> MTSHRQSSDTFGGILPSTLSSRYLSIVNQLPEEFSSVVSEMMVHLENIFSLAENFFQAIERFSRTPDLLERNKMSIGVGAEGDSWPCHVSHEAPMGSAQTTENSAKEEDKQVPESAALQHPKFKSTPGPQLPTRRRFLSESDELQDPQPVWDAEPQFCQGFLIQGLWELFMDSRQKNQQEHGGEDSSQESKDSGLCDFKPEPQPRHRNSLSDSADPFLIKSPSALLDYYQEDVSRPQPETQESSGRADKFLKPLSWGSEVLESSCNQPSTALWQLERFTVPQALQKVRVLKHQELLLVVAVSSFTRHVFTCSQSGIKVWNLVNQVAEDRDPESHLKCSVQDNKVYLRTCLLSSNSRTLFAGGYNLPGVIVWDLAAPSLYEKCQLPCEGLSCQALANTKENMALAGFTDGTVRIWDLRTQEIVRNLKGPTNSARNLVVKDDNIWTGGLDACLRCWDLR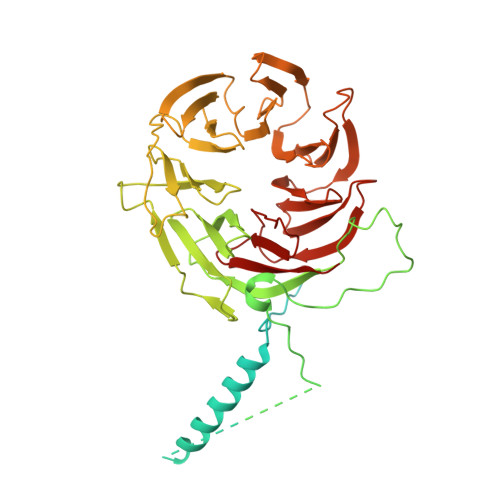MAKVSLEHLFQSQIMSLAHSPTEDWLLLGLANGQHCLFNSRKRDQVLTVDTKDNTILGLKFSPNGKWWASVGMGNFITVHSMPTGAKLFQVPEVGPVRCFDMTENGRLIITGSRDCASVYHIKY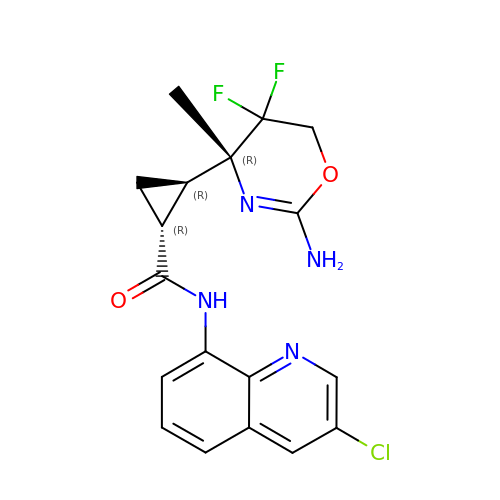(1~{R},2~{R})-2-[(4~{R})-2-azanyl-5,5-bis(fluoranyl)-4-methyl-6~{H}-1,3-oxazin-4-yl]-~{N}-(3-chloranylquinolin-8-yl)cyclopropane-1-carboxamide | C18 H17 Cl F2 N4 O2 | FPQSTKSVKJAHKE-PSTGCABASA-N Bacteria encode a variety of reverse transcriptases (RTs) that evolved from mobile group II intron RTs to perform different cellular functions. In a previous study, we showed via genetic and biochemical analyses that a Pseudomonas aeruginosa group II intron–like (G2L4) RT functions in DSBR via MMEJ both in its native host and when transferred into Escherichia coli. Here, we determined a 2.6-Å crystal structure of a full-length G2L4 RT apoenzyme and a 2.8-Å cocrystal structure of G2L4 RT bound in an active conformation to a snapback DNA synthesis substrate and incoming dNTP. All RTs share a common structural framework composed of fingers, palm, and thumb or thumb surrogate regions that fold into a hand-like structure, forming a cleft containing an RT active site composed of three conserved aspartate residues that bind catalytic Mg2+ ions.

Taking advantage of this activity, we obtained diffracting crystal of G2L4 RT bound to a 15-nt snapback DNA substrate (5’-AAGCGGTTAACCCAA-3’) that enabled initiation of DNA synthesis by base pairing of its two 3’ A residues (A14 and A15) to TT residues at upstream positions 7 and 8 (T7 and T8). To stabilize these short base-pairing interactions, the cocrystallization setup included Mn2+, which favors strand annealing by G2L4 RT, plus dCTP, and dideoxy GTP (ddGTP) to enable addition of three complementary nucleotides at positions +1 to +3 ending with ddGTP and followed by base pairing of an incoming dCTP opposite the templating base (G3 at position −1 in the snapback substrate). To solve the structure, we defined the fingers/palm and thumb as separate rigid bodies during molecular replacement to allow mobility between these two regions. This led to a solution in space group P212121, revealing a G2L4 RT dimer with each monomer bound to a separate 15-nt snapback DNA substrate per asymmetric unit. The intervening AACCC loop (nucleotides 9 to 13) was not visible in the structure and presumably disordered. Because dCTP and ddGTP were included in the crystallization solution, two C residues complementary to G5 and G6 and ddGTP complementary to C4 of the template were added to the 3’ end of the DNA substrate, stabilizing the annealed microhomology. dCTP complementary to G3 was bound at the active site but not incorporated due to lack of free hydroxyl groups on the preceding 3’-terminal dideoxyguanosine. Compared to its occluded apoenzyme structure, each G2L4 RT monomer adopted an active configuration with the NTE moving outward to accommodate the bound DNA and the bound DNA substrate pushing the RT3a plug completely out of the active site. Extrusion of the RT3a plug allowed the disordered RT1 in the apoenzyme structure to form the expected antiparallel β-strands over the active-site pocket as in other RTs and the AQG motif to revert to its functional position to coordinate alignment of the incoming dNTP, resulting in an active structure similar to that of GII RT.

>[2x]SRLYKDICSLRTLYGAWRKVRSSAFLSSSDEIRREAEEFESRLPDSLIEIQHALSKQIFIFLQQTGVAQKKPGGKSRPLVLAPIPNRVVQRALLDVLQRRVRLVKRVLGTPTSYGGIPDKRVAMAIADAREAMRTGARFHIRSDIPAFFTKINKDRVLELLRPHLNCEATLKLFEEAIRTDLANIDDLRRKGLDEIFPIGIEGVAQGSPLSPLLANIYLADFDLAMNSNGITCLRYIDDFLLLGASLSDVDKAFNRALKELGKIGLEAYDPRTDKTKASRGATEIGFDFLGCNVSPGLIQPSEATRRRFRAKLDAEFVAASHALRYNAQYQDGDGKYSYSSALYRIDKIILGWGKAFTFCNGSQCMIALDDFISNKLAQLEAEKIAILANSDSTVRRRVLGVRLLIDI> GGCGAUAUGGCAUGGAAUCAGCUCAAGGAACUGUGAACGUAUAUCGGGCA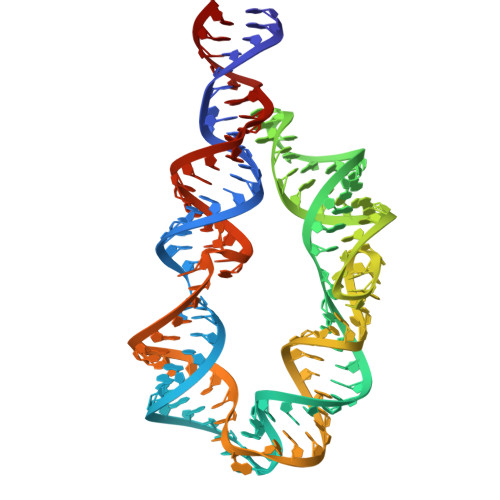ACGACUAGGAAACUAGUCGUUGGGAAGAAACUGCCGAUAUACGGGAGUUCCUUGAGCGGGAGAUUCCAUGCCUAAGUCGC> MSAAPVLSITNASVVYPDGISTVTALDSANVEIFPGELVAIVGESGSGKSTLLSIAGFLQEPTSGTVTLHGAEGLDATSTRREHIGFVFQQPNLLGSLTAREQLLITDHLRGIKPRKDRADELLARVGLKGLGGRRVAQLSGGQRQRVNIARALMGNPQLLLADEPTSALDARLSKEIVELLRDVTKEFALATLMVTHDRSQLAYADRFVEMADGKALQTAKLWSHPQFEK;> MFLGIRDIRAAAGRFALIASVVGLITLLIVMLTGLTQGLGKQNTSAIEALAPHSVVFTTAGGSSPEFTSSEISEQQAERWKDSTPLGVSQTRIESDQNANTTAVMGLPEGTPLPDSVGGFIEQGALLPAELADFLHVRAGDHITLGGATVTVAGTVKTENYSHTPVVWVDTATWQLVSHTKAVGTVLLLNQEPTIQPQDNEVVTDLKGAFQAMPAYK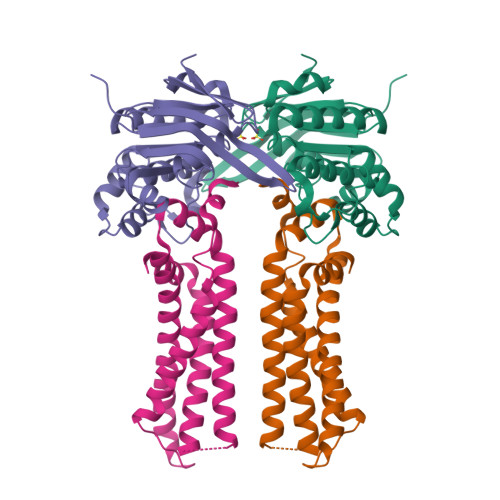SERSSLLSMQAFLYIISALVTVAFLTVWTLQRTRDIAVLAALGASKRYLLIDALGQAAIILAAGVALGAGIGALLGWLIAGSVPFSLGWVSVLGPALGIWLLGLIGATIAVRNVTKVDPQIALGATA>[4x]MENTENSVDSKSIKNLEPKIIHGSESMDSGISLDNSYKMDYPEMGLCIIINNKNFHKSTGMTSRSGTDVDAANLRETFRNLKYEVRNKNDLTREEIVELMRDVSKEDHSKRSSFVCVLLSHGEEGIIFGTNGPVDLKKITNFFRGDRCRSLTGKPKLFIIQACRGTELDCGIETD;>SGVDDDMACHKIPVEADFLYA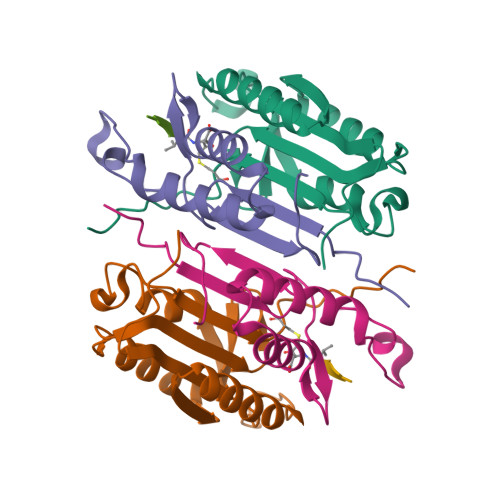YSTAPGYYSWRNSKDGSWFIQSLCAMLKQYADKLEFMHILTRVNRKVATEFESFSFDATFHAKKQIPCIVSMLTKELYFYHHHHHH[4x]>GAMAETVFKQNHAASGFLAGRYDAQAMSPTMFNWSRESRFTSTADGALKWEKNVPATPQNGAGAAVDGDGTVFIQSKDGKLTAYHPDGTVKWVTENLGTTYTLTPVLGTNGVIYLPSHDKKLYFID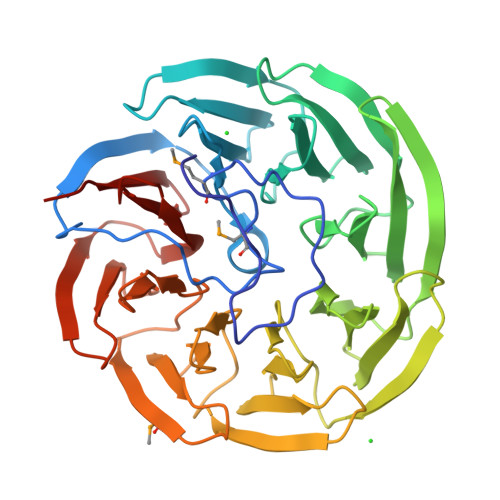KETGNILTSVPLSGAPSSDAAIGPDGTLYVSTLDNYIYAIKPTSPSTWTQKWKFKTNGVVGSAPVLASNGTLYTATYNNIFYAINSGTGQVKWSKTTSNGFKGYPVIDRDGTVYAGNQDGNLYAYTSTGAVKWTFPLNGFSSSSLAIDHNGNVYIGSGSGELFSISKTGNMNWSFYTDGPVRTAPLIDADGNVYFGSDDKNVYAVDADGNEKWRYQTDSNVISSPVLAEDGTLYVGTYTKLLAFGAKK[2x]> RDHFALDRPSETHADYLLRTGQVVDISDTIYPRNPAMYCEEARLKSFQNWPDYAHLTPREL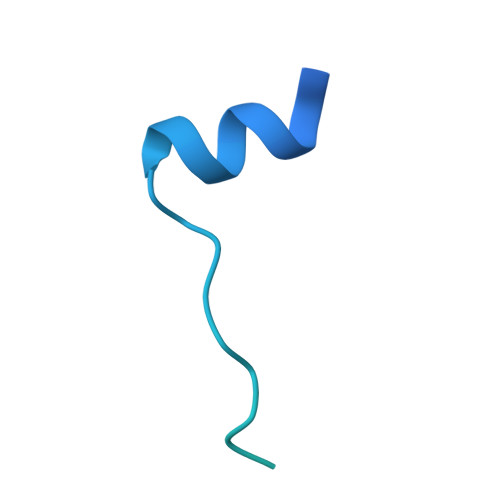ASAGLYYTGIGDQVQCFCCGGKLKNWEPCDRAWSEHRRHFPNCFFVLGRNLNIRSE>MFRPLPITLQRGALRLEPMVEADVPELVELADANREVLQYMSAPQRPDWYRQAIADQREGRALPLVVRLGNRIVGTTRFLDFMPALPACEIGGTWLEQSQHGMGLNASMKYLMLR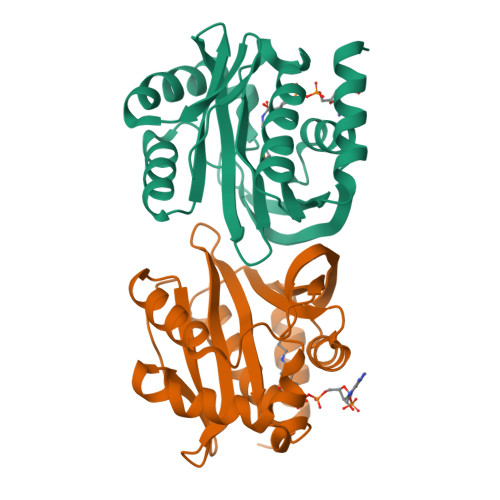HAFDSWQMVRVQLKTAASNLRSQRAIEKLGAVREGVLRNHRRLAGGRLDDSVLYSITDHEWPQVKAALEAGFSG[4x]>[2x]MPNFAGTWKMRSSENFDELLKALGVNAMCRKVAVAAASKPHVEIRQDGDQFYIKTSTTVRTTEINFKVGEGFEEETVDGRKCRSLATWENENKIHCTQTLLEGDGPKTYWTRELANDE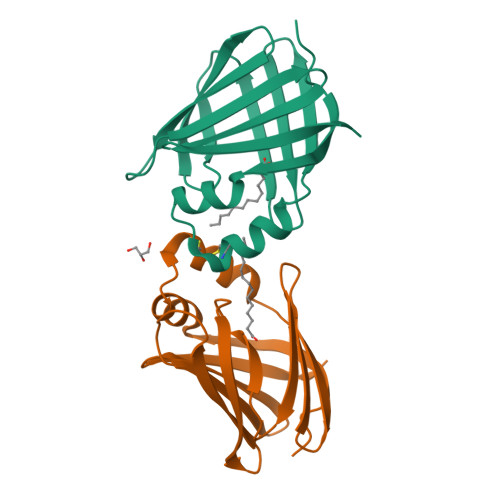LILTFGADDVVCTRIYVRE> YNPRKFSEKIALQKQRQAEETAAFEEVMM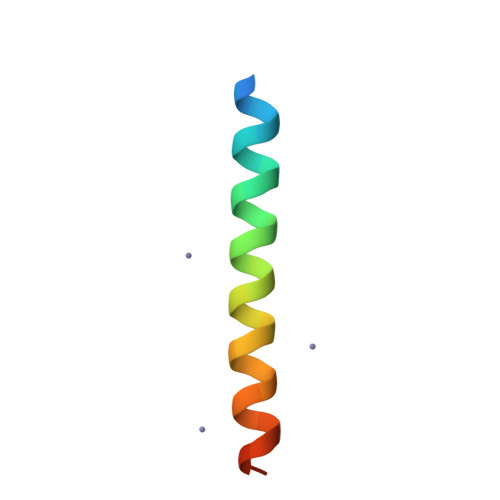DIGST> RGSHHHHHHGSALLAEHLLRPLPADKQIETGPFLEAVSHLPPFFDCLGSPVFTPIKADISGNITKIKAVYDTNPTKFRTLQNILEVEKEMYGAEWPKV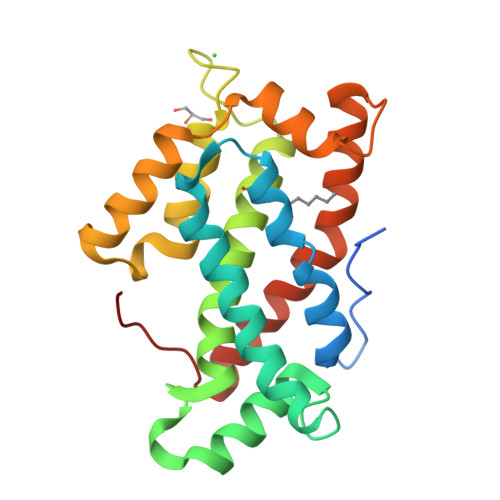GATLALMWLKRGLRFIQVFLQSICDGERDENHPNLIRVNATKAYEMALKKYHGWIVQKIFQAALYAAPYKSDFLKALSKGQNVTEEECLEKVRLFLVNYTATIDVIYEMYTRMNAELNYKV> GSLDALGSQPIHLWQFLKELLLKPHSYGRFIRWLNKEKGIFKIE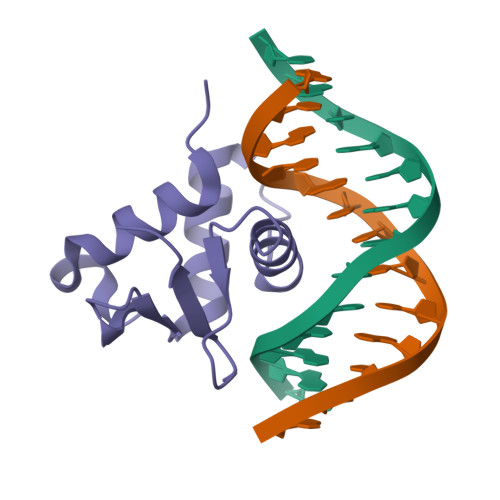DSAQVARLWGIRKNRPAMNYDKLSRSIRQYYKKGIIRKPDISQRLVYQFVHPI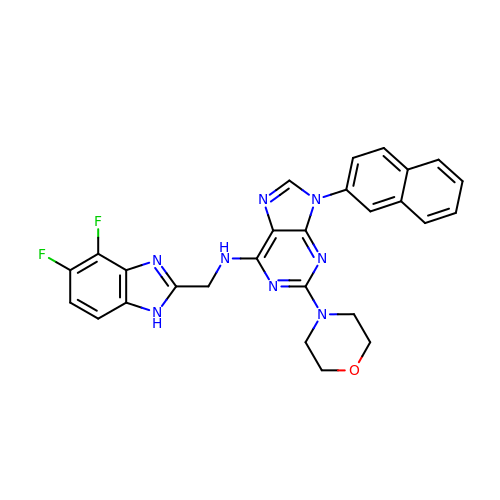~{N}-[[4,5-bis(fluoranyl)-1~{H}-benzimidazol-2-yl]methyl]-2-morpholin-4-yl-9-naphthalen-2-yl-purin-6-amine | C27 H22 F2 N8 O | DOPHVIBXJOSQHB-UHFFFAOYSA-N> MGSSHHHHHHSQDPMVL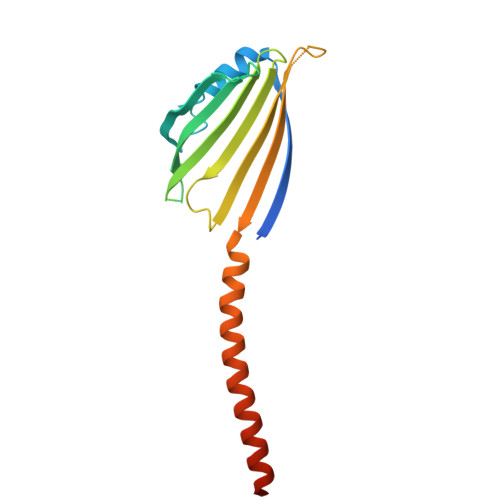LHKSTHIFPTDFASVSRAFFNRYPNPYSPHVLSIDTISRNVDQEGNLRTTRLLKKSGKLPTWVKPFLRGITETWIIEVSVVNPANSTMKTYTRNLDHTGIMKVEEYTTYQFDSATSSTIADSRVKFSSGFNMGIKSKVEDWSRTKFDENVKKSRMGMAFVIQKLEEARNPQF> GGUCAAGAUAGUAAGGGUCCACGGUGGAUGCCCUGGCGCUGGAGCCGAUGAAGGACGCGAUUACCUGCGAAAAGCCCCGACGAGCUGGAGAUACGCUUUGACUCGGGGAUGUCCGAAUGGGGAAACCCACCUCGUAAGAGGUAUCCGCAAGGAUGGGAACUCAGGGAACUGAAACAUCUCAGUACCUGAAGGAGAAGAAAGAGAAUUCGAUUCCGUUAGUAGCGGCGAGCGAACCCGGAUCAGCCCAAACCGAAACGCUUGCGUUUCGGGGUUGUAGGACCAGUUUUUAAGAUUCAACCCCUCAAGCCGAAGUGGCUGGAAAGCUACACCUCAGAAGGUGAGAGUCCUGUAGGCGAACGAGCGGUUGACUGUACUGGCACCUGAGUAGGUCGUUGUUCGUGAAACGAUGACUGAAUCCGCGCGGACCACCGCGCAAGGCUAAAUACUCCCAGUGACCGAUAGCGCAUAGUACCGUGAGGGAAAGGUGAAAAGAACCCCGGGAGGGGAGUGAAAGAGAACCUGAAACCGUGGACUUACAAGCAGUCAUGGCACCUUAUGCGUGUUAUGGCGUGCCUAUUGAAGCAUGAGCCGGCGACUUAGACCUGACGUGCGAGCUUAAGUUGAAAAACGGAGGCGGAGCGAAAGCGAGUCCGAAUAGGGCGGCAUUAGUACGUCGGGCUAGACUCGAAACCAGGUGAGCUAAGCAUGACCAGGUUGAAACCCCCGUGACAGGGGGCGGAGGACCGAACCGGUGCCUGCUGAAACAGUCUCGGAUGAGUUGUGUUUAGGAGUGAAAAGCUAACCGAACCUGGAGAUAGCUAGUUCUCCCCGAAAUGUAUUGAGGUACAGCCUCGGAUGUUGACCAUGUCCUGUAGAGCACUCACAAGGCUAGGGGGCCUACCAGCUUACCAAACCUUAUGAAACUCCGAAGGGGCACGCGUUUAGUCCGGGAGUGAGGCUGCGAGAGCUAACUUCCGUAGCCGAGAGGGAAACAACCCAGACCAUCAGCUAAGGUCCCUAAAUGAUCGCUCAGUGGUUAAGGAUGUGUCGUCGCAUAGACAGCCAGGAGGUUGGCUUAGAAGCAGCCACCCUUCAAAGAGUGCGUAAUAGCUCACUGGUCGAGUGACGAUGCGCCGAAAAUGAUCGGGGCUCAAGUGAUCUACCGAAGCUAUGGAUUCAACUCGCGAAGCGAGUUGUCUGGUAGGGGAGCGUUCAGUCCGCGGAGAAGCCAUACCGGAAGGAGUGGUGGAGCCGACUGAAGUGCGGAUGCCGGCAUGAGUAACGAUAAAAGAAGUGAGAAUCUUCUUCGCCGUAAGGACAAGGGUUCCUGGGGAAGGGUCGUCCGCCCAGGGAAAGUCGGGACCUAAGGUGAGGCCGAACGGCGCAGCCGAUGGACAGCAGGUCAAGAUUCCUGCACCGAUCAUGUGGAGUGAUGGAGGGACGCAUUACGCUAUCCAAUGCCAAGCUAUGGCUAUGCUGGUUGGUACGCUCAAGGGCGAUCGGGUCAGAAAAUCUACCGGUCACAUGCCUCAGACGUAUCGGGAGCUUCCUCGGAAGCGAAGUUGGAAACGCGACGGUGCCAAGAAAAGCUUCUAAACGUUGAAACAUGAUUGCCCGUACCGCAAACCGACACAGGUGUCCGAGUGUCAAUGCACUAAGGCGCGCGAGAGAACCCUCGUUAAGGAACUUUGCAAUCUCACCCCGUAACUUCGGAAGAAGGGGUCCCCACGCUUCGCGUGGGGCGCAGUGAAUAGGCCCAGGCGACUGUUUACCAAAAUCACAGCACUCUGCCAACACGAACAGUGGACGUAUAGGGUGUGACGCCUGCCCGGUGCCGGAAGGUCAAGUGGAGCGGUGCAAGCUGCGAAAUGAAGCCCCGGUGAACGGCGGCCGUAACUAUAACGGUCCUAAGGUAGCGAAAUUCCUUGUCGGGUAAGUUCCGACCUGCACGAAAGGCGUAACGAUCUGGGCGCUGUCUCAACGAGGGACUCGGUGAAAUUGAAUUGGCUGUAAAGAUGC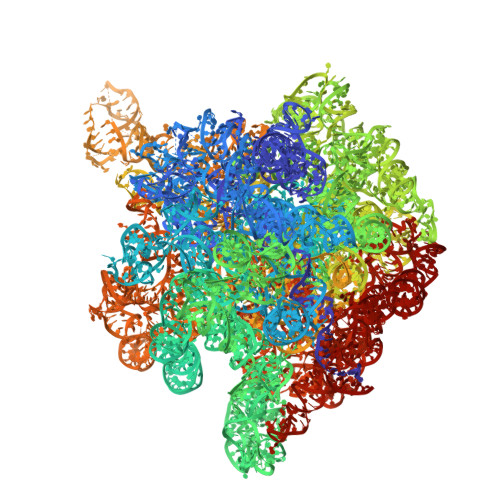GGCCUACCCGUAGCAGGACGAAAAGACCCCGUGGAGCUUUACUAUAGUCUGGCAUUGGGAUUCGGGUUUCUCUGCGUAGGAUAGGUGGGAGCCUGCGAAACUGGCCUUUUGGGGUCGGUGGAGGCAACGGUGAAAUACCACCCUGAGAAACUUGGAUUUCUAACCUGAAAAAUCACUUUCGGGGACCGUGCUUGGCGGGUAGUUUGACUGGGGCGGUCGCCUCCCAAAAUGUAACGGAGGCGCCCAAAGGUCACCUCAAGACGGUUGGAAAUCGUCUGUAGAGCGCAAAGGUAGAAGGUGGCUUGACUGCGAGACUGACACGUCGAGCAGGGAGGAAACUCGGGCUUAGUGAACCGGUGGUACCGUGUGGAAGGGCCAUCGAUCAACGGAUAAAAGUUACCCCGGGGAUAACAGGCUGAUCUCCCCCGAGAGUCCAUAUCGGCGGGGAGGUUUGGCACCUCGAUGUCGGCUCGUCGCAUCCUGGGGCUGAAGAAGGUCCCAAGGGUUGGGCUGUUCGCCCAUUAAAGCGGCACGCGAGCUGGGUUCAGAACGUCGUGAGACAGUUCGGUCUCUAUCCGCUACGGGCGCAGGAGAAUUGAGGGGAGUUGCUCCUAGUACGAGAGGACCGGAGUGAACGGACCGCUGGUCUCCCUGCUGUCGUACCAACGGCACAUGCAGGGUAGCUAUGUCCGGAACGGAUAACCGCUGAAAGCAUCUAAGCGGGAAGCCAGCCCCAAGAUGAGUUCUCCCACUGUUUAUCAGGUAAGACUCCCGGAAGACCACCGGGUUAAGAGGCCAGGCGUGCACGCAUAGCAAUGUGUUCAGCGGACUGGUGCUCAUCAGUCGAGGUCUUGACCACUC> DSLRPKLSEEQQRIIAILLDAHHKTYDPTYSDFCQFRPPVRVNDGGGSHPSRPNSRHTPSFSGDSSSSCSDHCITSSDMMDSSSFSNLDLSEEDSDDPSVTLELSQLSMLPHLADLVSYSIQKVIGFAKMIPGFRDLTSEDQIVLLKSSAIEVIMLRSNESFTMDDMSWTCGNQDYKYRVSDVTK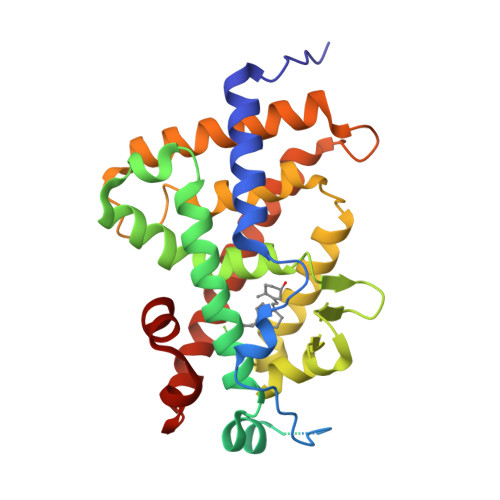AGHSLELIEPLIKFQVGLKKLNLHEEEHVLLMAICIVSPDRPGVQDAALIEAIQDRLSNTLQTYIRCRHPPPGSHLLYAKMIQKLADLRSLNEEHSKQYRCLSFQPECSMKLTPLVLEVFG> GSHMIQAYLGLGSNIGDRESQLNDAIKILNEYDGISVSNISPIYETAPVGYTEQPNFLNLCVEIQTT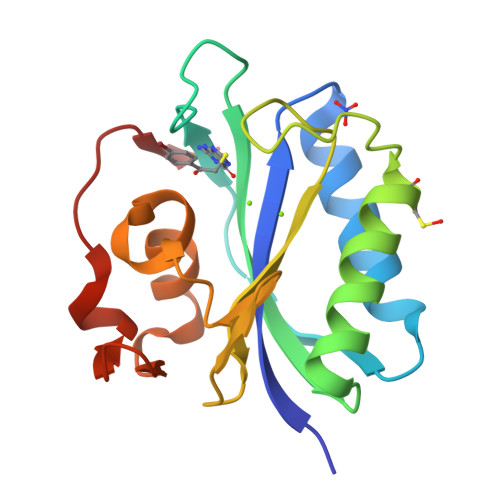LTVLQLLECCLKTEECLHRIRKERWGPRTLDVDILLYGEEMIDLPKLSVPHPRMNERAFVLIPLNDIAANVVEPRSKLKVKDLVFVDDSVKRYK HOs catalyze the oxidative cleavage of heme to biliverdin, carbon monoxide, and ferrous iron, in a reaction that proceeds via a complex multistep mechanism. The HO enzyme present in L. interrogans (LepHO) is required for iron utilization when hemoglobin is the sole iron source and is an important virulence factor in the hamster model of infection. We also showed that the redox partner of LepHO is a ferredoxin-NADP+ reductase (LepFNR), a plastidic-type enzyme found in this bacterium. Hence, the catalytic heme degradation supported by LepHO and its cognate electron transfer partner enables L. interrogans cells to utilize iron from host heme and provide a mechanism for circumventing the iron-limitation conditions imposed by the host defense system.

Herein we report the crystal structure of LepHO-heme at 1.73 Å resolution, which displays distinct features compared to the structures of other structurally characterized HOs. To this end, the LepHO-C26S-stop variant was generated by introducing two mutations; the codon for residue E206 was replaced with a stop signal, and the codon for the C26 was replaced by one coding for serine. From these data, it can be concluded that neither the replacement of C26 by serine nor the removal of the 20 residues from the C-terminal, significantly alter the capability of the enzyme to degrade heme. The folding of LepHO is similar to that of other known HOs; it consists of a single domain of approximately 50 x 40 x 35 Å composed mostly of α-helices. The heme is sandwiched between the proximal and distal helices, and the heme-iron is axially coordinated by the Nε2 nitrogen atom of H15, which resides in the proximal helix and by a water molecule in the distal site. Analysis of the electron density in our crystallographic structure allowed us to corroborate the heme seating predicted from the 1H NMR analysis, as well as the presence of both heme isomers in LepHO. In LepHO, G128 is within hydrogen bond distance (2.85 Å) of a water molecule in the distal site near the heme. A relatively rigid network of water molecules, which extends from the active site to the surface of the enzyme, is also present in the crystal structure of LepHO. H40 in LepHO hydrogen bonds a water molecule in the network, a function that is usually carried out by an aspartate in other HOs. Analysis of the LepHO structure revealed that residues F157 and I160 are part of a depression on the enzyme surface which likely constitutes the outermost section lining the network of hydrogen bonded waters, or said in other words, the probable entrance to the network from the aqueous environment.

> GHMASGSMSLATILREGTSEEHKAAESSAFIRSFMKGILEKGTYARHLEAFYYVYESMEEELERNKNNLVLKSIYFPELYRKNALLEDLQFFYGTWKPNDHQPSVATQDYVQRIRKISETQPELLAAHSYVRYLGDLSGGQILKKVAARALNLPEGKGISFYEFPMIQDINGFKQNYRTALDSLPVNDSEKQSILAESKQVFLLNQGIFSEL> G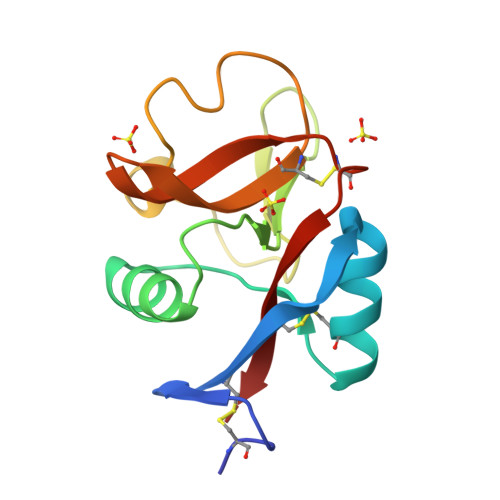SCPKDWKPFVSHCYFILNDSKASWNESEEKCSHMGAHLVVIHSQAEQDFITSNLNTSAGYFIGLLDAGQRQWRWIDQTPYNKSATFWHKGEPNQDWERCVIINHKTTGWGWNDIPCKDEHNSVCQVKK>[4x]MLVEGSELQSGAQQPRTEAPQHGELQYLRQVEHIMRCGFKKEDRTGTGTLSVFGMQARYSLRDEFPLLTTKRVFWKGVLEELLWFIKGSTNAKELSSKGVRIWDANGSRDFLDSLGFSARQEGDLGPVYGFQWRHFGADYKDMDSDYSGQGVDQLQKVIDTIKTNPDDRRIIMCAWNPKDLPLMALPPCHALCQFYVVNGELSCQLYQRSGDMGLGVPFNIASYALLTYM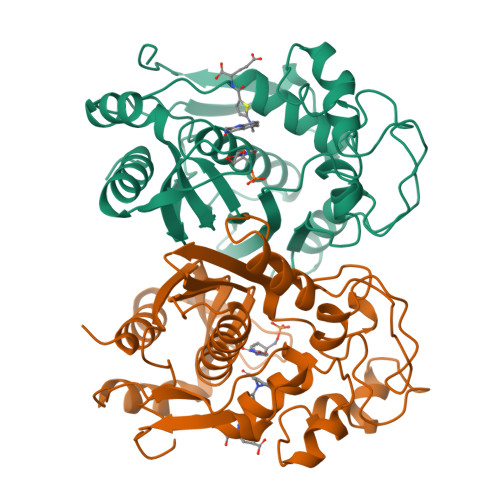IAHITGLQPGDFVHTLGDAHIYLNHIEPLKIQLQREPRPFPKLRILRKVETIDDFKVEDFQIEGYNPHPTIKMEMAV>[2x]ASSTNLKDVLASLIPKEQARIKTFRQQHGNTAVGQITVDMSY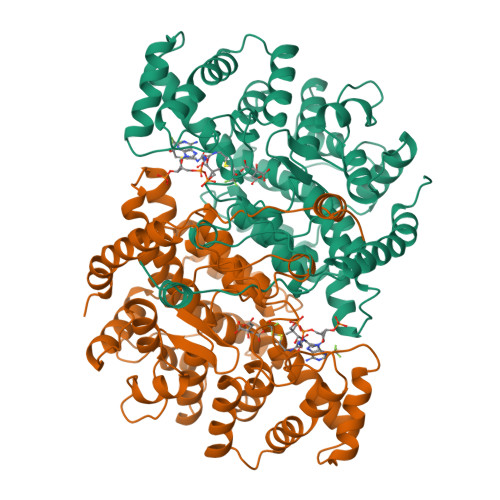GGMRGMKGLIYETSVLDPDEGIRFRGFSIPECQKLLPKAGGGEEPLPEGLFWLLVTGQIPTPEQVSWVSKEWAKRAALPSHVVTMLDNFPTNLHPMSQLSAAITALNSESNFARAYAEGINRTKYWEFVYEDAMDLIAKLPCVAAKIYRNLYRAGSSIGAIDSKLDWSHNFTNMLGYTDPQFTELMRLYLTIHSDHEGGNVSAHTSHLVGSALSDPYLSFAAAMNGLAGPLHGLANQEVLLWLSQLQKDLGADASDEKLRDYIWNTLNSGRVVPGYGHAVLRKTDPRYTCQREFALKHLPSDPMFKLVAQLYKIVPNVLLEQGKAKNPWPNVDAHSGVLLQYYGMTEMNYYTVLFGVSRALGVLAQLIWSRALGFPLERPKSMSTAGLEKLSAGG> MTASPDYLVVLFGITAGATGAKLGSDEKELILLFWKVVDLANKKVGQLHEVLVRPDQLELTEDCKEETKIDVESLSSASQLDQALRQFNQSVSNELNIGVGTSFCLCTDGQLHVRQILHPEASKKNVLLPECFYSFFDLRKEFKKCCPGSPDIDKLDVATMTEYLNFEKSSSVSRYGASQVEDMGNIILAMISEPYNHRFSDPERVNYKFESGTCSKMELIDDNTVVRARGLPWQSSDQDIARFFKGLNIAKGGAALCLNAQGRRNGEA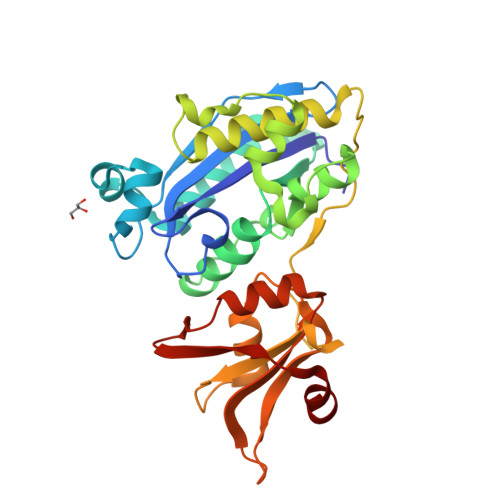LVRFVSEEHRDLALQRHKHHMGTRYIEVYKATGEDFLKIAG> MNKVIVAAFVSAFVLGSTATFASGNLESSLAPISAKDMLDYLACKDKKPTDVVKSHTEVENGKIVRVKCGD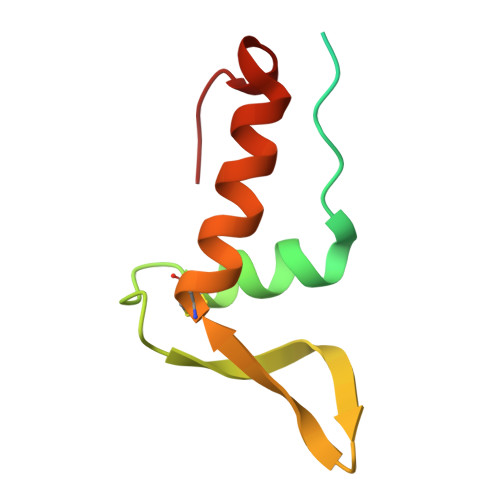IVALVQKAREQSGDAWQGGY> GESQED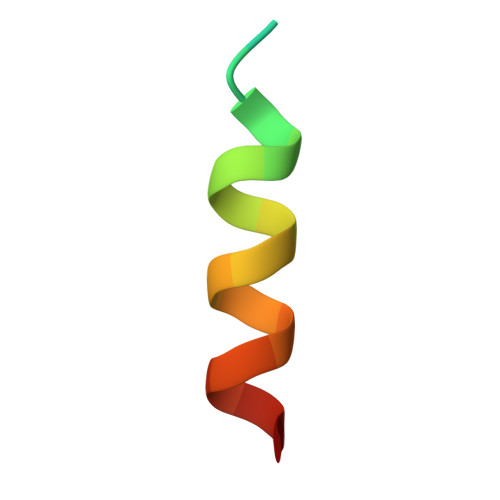MFAKLKEKFFNEINK> MAHHHHHHMTEIDDLLRKNPELQKEWKRTVWTAAISSGVIAYRPPLLERAFREFPMETAKSALNLFVAAHKSKNRQSVDIITQNLKDAKTFPLGQLEEEIVTDILKYPNLLEKLLQTGWNPNLILEWEKHKSLSQNSKRSHRRPEILIKSNGKEFIEKQETTLLILAMQNDFIPMETVQILLKYGADP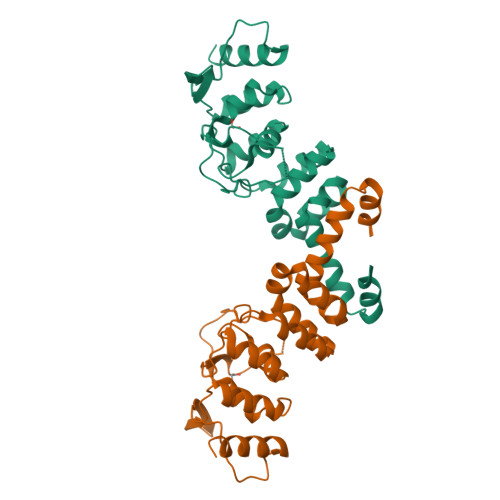SLGVKRKSEGKEYLLYPLANINSNGNTILKELKQKTLIDWKK> DRMVMGKIKRIEAGLPLTTAKGRTFGYDVIDTKLYINEEEAKQLRLIYDIFEEEQSITFLQKRLKKLGFKVRTYNRYNNWLTNDLYCGYVSYKDKVHVKGIHEPI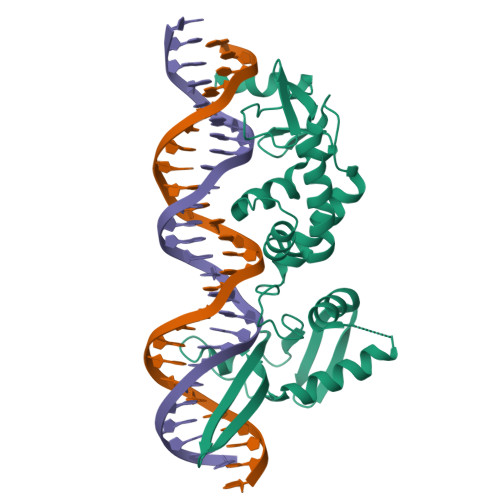ISEEQFYRVQEIFSRMGKNPNMNKESASLLNNLVVCSKCGLGFVHRRKDTVSRGKKYHYRYYSCKTYKHTHELEKCGNKIWRADKLEELIIDRVNNYSFASRNIDKEDELDSLNEKLKIEHAKKKRLFDLYINGSYEVSELDSMMNDIDAQINYYEAQIEANEELKKNKKIQENLADLATVDFNSLEFREKQLYLKSLINKIYIDGEQVTIEWL2,6-DIMETHYL-7-OCTEN-2-OL | C10 H20 O | 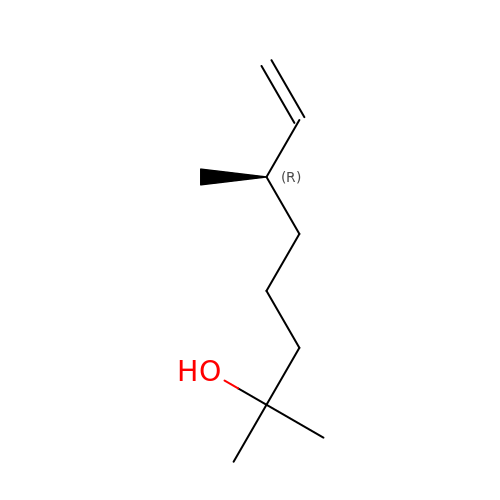XSNQECSCDATQEL-VIFPVBQESA-N> DPTQFEERHLKFLQQLGKGNFGSVEMCRYDPLQDNTGEVVAVKKLQHSTEEHLRDFEREIEILKSLQHDNIVKYKGVCYSAGRRNLKLIMEYLPYGSLRDYLQKHKERIDHIKLLQYTSQICKGMEYLGTKRYIHRDLATRNILVENENRVKIGDFGLTKVLPQDKEYYKVKEPGESPIFWYAPESLTESKFSVASDVWSFGVVLYELFTYIEKSKSPPAEFMRMIGNDKQGQMIVFHLIELLKNNGRLPRPDGCPDEIYMIMTECWNNNVNQRPSFRDLALRVDQ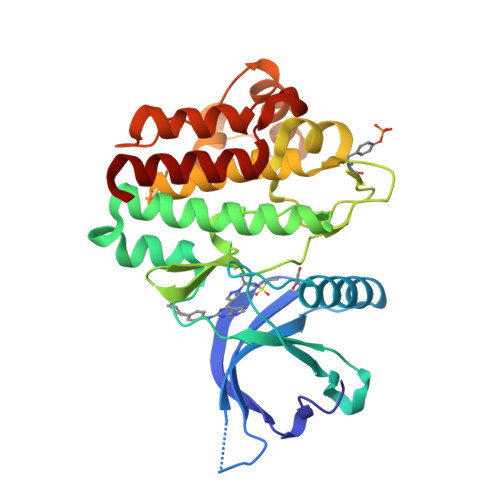IRDNMAG>KSQIKRQKMIYHCKFGEFGVMEGQFTEPSGVAVNAQNDIIVADTNNHRIQIFDKEGRFKFQFGECGKRDSQLLYPNRVAVVRNSGDIIVTERSPTHQIQIYNQYGQFVRKFGATILQHPRGVTVDNKGRIIVVECKVMRVIIFDQNGNVLHKFGCSKHLEFPNGVVVNDKQEIFISDNRAHCVKVFNYEGQYLRQIGGEGITNYPIGVGINSNGEILIADNHNNFNLTIFTQDGQLI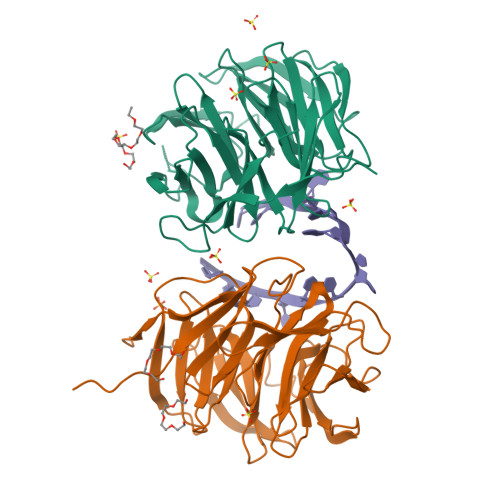SALESKVKHAQCFDVALMDDGSVVLASKDYRLYIYRYVQLAPVGM[2x]> VDERNECGQTPLMIAAEQGNLEIVKELIKNGANCNLEDLDNWTALISASKEGHVHIVEELLKCGVNLEHRDMGGWTALMWACYKGRTDVVELLLSHGANPSVTGLYSVYPIIWAAGRGHADIVHLLLQNGAKVNCSDKYGTTPLVWAARKGHLECVKHLLAMGADVDQEGANSMTALIVAVKGGYTQSVKEILKRNPNVNLTDKDGNTALMIASKEGHTEIVQDLLDAGTYVNIPDRSGDTVLIGAVRGGHVEIVRALLQKYADIDIRGQDNKTALYWAVEKGNATMVRDILQCNPDTEICTKDGETPLIKATKMRNIEVVELLLDKGAKVSAVDKKGDTPLHIAIRGRSRKLAELLLRNPKD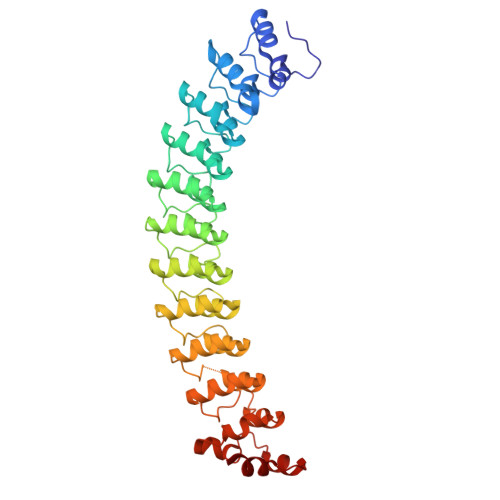GRLLYRPNKAGETPYNIDCSHQKSILTQIFGAR> QGVNDNEEGFFSARGHRPLDKKREEAPSLRPAPPPISGGGYRARPAKAAATQKKVERKAPDAG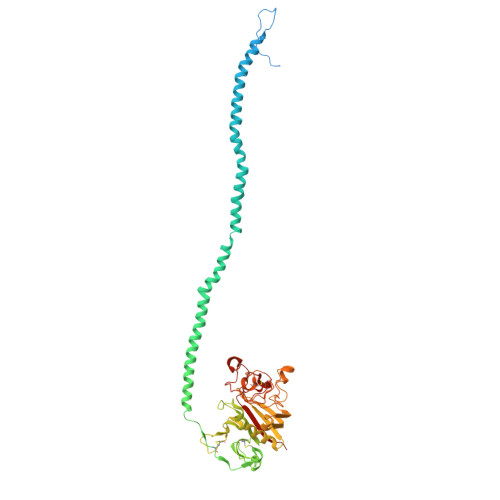GCLHADPDLGVLCPTGCQLQEALLQQERPIRNSVDELNNNVEAVSQTSSSSFQYMYLLKDLWQKRQKQVKDNENVVNEYSSELEKHQLYIDETVNSNIPTNLRVLRSILENLRSKIQKLESDVSAQMEYCRTPCTVSCNIPVVSGKECEEIIRKGGETSEMYLIQPDSSVKPYRVYCDMNTENGGWTVIQNRQDGSVDFGRKWDPYKQGFGNVATNTDGKNYCGLPGEYWLGNDKISQLTRMGPTELLIEMEDWKGDKVKAHYGGFTVQNEANKYQISVNKYRGTAGNALMDGASQLMGENRTMTIHNGMFFSTYDRDNDGWLTSDPRKQCSKEDGGGWWYNRCHAANPNGRYYWGGQYTWDMAKHGTDDGVVWMNWKGSWYSMRKMSMKIRPFFPQQ>[2x]GSYDSSSSSSNDSSARNEEDESCMFA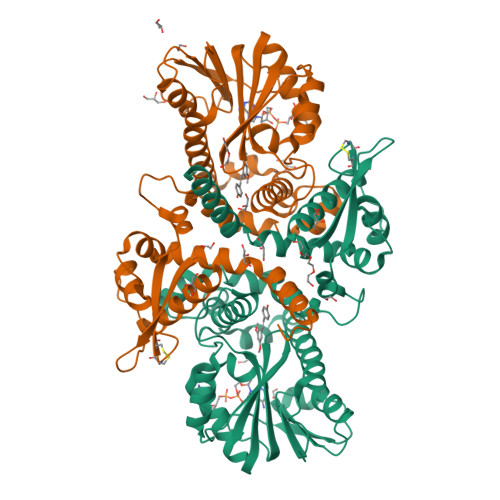LKLLGGFAVPFTIKAVIELGVMDQLLTAERAMSAEELVAAAVAAQLPRPEVACTMVDRLLRFLASHSVVRCTTEVVVGTDDATTTTCCRRSYAASPVCKWFARNGVEDSVLPLGMMILNKTFLDSWQNITDAVLEGAAPFEKTYGMPMFEYLSTNGPLNTVFHEAMANHSMIITKKLLKFFRGFEGLDVLVDVGGGNGTTLQMIRGQYKNMRGINYDLPHVIAQAAPVEGVEHVGGSMFDNIPRGNAVLLKWILHDWDDKACIKILKNCYTALHVRGKVIVLEYVVPDEPEPTLAAQGAFELDLTMLVTFGSGKERTQREFSELAMEAGFSREFKATYIFANVWALEFTK> KETCSTGLYTHSGECCKACNLGEG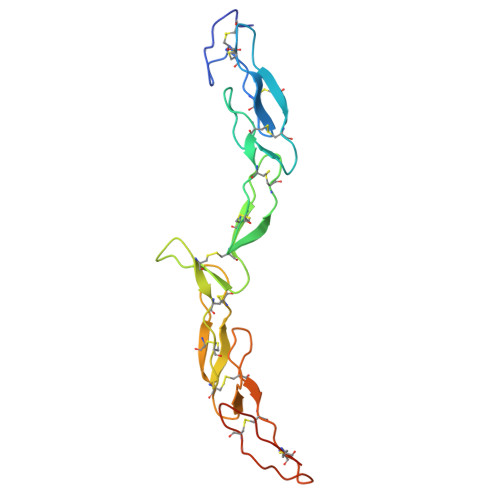VAQPCGANQTVCEPCLDSVTFSDVVSATEPCKPCTECLGLQSMSAPCVEADDAVCRCAYGYYQDEETGHCEACSVCEVGSGLVFSCQDKQNTVCEECPEGTYSDEANHVDPCLPCTVCEDTERQLRECTPWADAECEHHHHHH>GPLGSATITQDTPINQIFTDTALAEKMKTVLGKTNVTDTVSQTDLDQVTTLQADRLGIKSIDGVEYLNNLTQINFSNNQLTDITPLKNLTKLVDILMNNNQIADITPLANLTNLTGLTLFNNQITDIDPLKNLTNLNRLELSSNTISDISALSGLTSLQQLSFGNQVTDLKPLANLTTLERLDISSNKVSDISVLAKLTNLESLIATNNQISDITPLGILTNLDELSLNGNQLKDIGTLASLTNLTDLDLANNQISNLAPLSGLTKLTELKLGANQISNISPLAGLTALTNLELNENQLEDISPISNLKNLTYLTLYFNNISDISPVSSLTKLQRLFFYNNKVSDVSSLANLTNINWLSAGH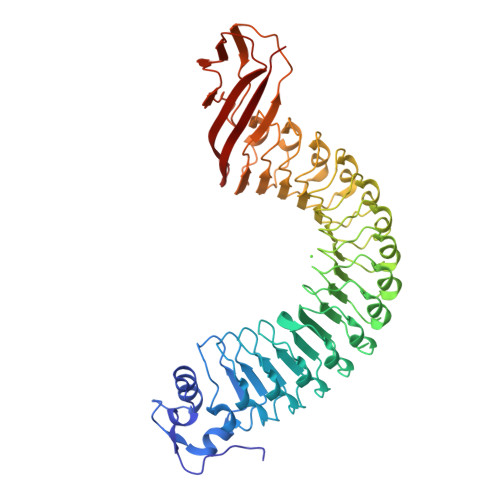NQISDLTPLANLTRITQLGLNDQAWTNAPVNYKANVSIPNTVKNVTGALIAPATISDGGSYTEPDITWNLPSYTNEVSYTFSQPVTIGKGTTTFSGTVTQPLKA[2x]>[6x]MSGPNYVMHTNDGRSIVTDGKPQTDNDTGMISYKDANGNKQQI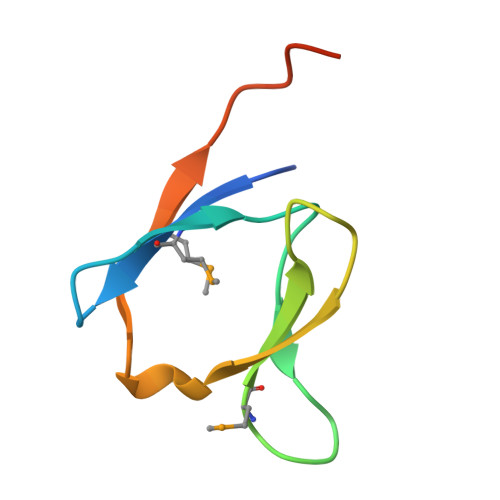NRTDVKEMVALENLEHHHHHH>[2x]MRVFHFSKLPLGVAILAASSSVFAVTLDGGAVAAPDQYGAKVAAEILKKGGNAVDAAVATAFTLAVTYPEAGNIGGGGFMTLYVDGKPYFLDYREIAPKAATKTMYLNEKGEVIENLSLVGAKAAGVPGTVMGLWEAHQRFGKLKWSELLTPAIGYAQTGFKVADQQYQYRQDAIALFNGKTNFGDYFGTMKPGEVFKQPELAKTLERIADKGPDDFYKGETAKLLIAQMKQDGGLITSDDLVDYQAKWREPMRIDWQGNTLYTAPLPSSGGIALAQLIGIKEQRAADFKGVELNSAKYIHLLSEIEKRVFADRADYLGDPQFSKVPVAQLTDPKYIAKRAGEVNPDAISATEKVRPGLEPHQTTHFSIVD;>TTHFSIVDKDGNAVSNTYTLNWDFGSGVVVKGAGFLLNDEMDDFSSKPGVANAFGVVGSDANAIEPGKRMLSSMSPSIVTRDGHVSLVLGTPGGSRIFTSIFQVLNNVYDFHLPLEKAVAAQRVHHQLLPK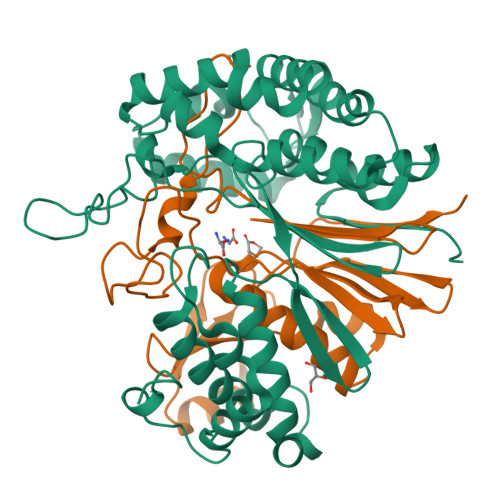DTIYYDAYAPLTGKVADELKAMGYTLEDQGDNMGDIQAIRVNGKALETASDPRGRGVGMVVKP[2x]>MDDANSSDSKVLNVWAMGDEAKSLKELAQKFTKDTGIEVKVQVIPWANAHDKLLTAVASKSGPDVVQMGTTWMPEFVEAGALLDITKDVEKSKNMNSDLFFPGSVKTTQFDGKTYGVPWYAETRVLFYRTDLLKKVGYNEAPKTWDELSDAALKLSKRGKDMYGFAIDPNEQTTGFIFGRQNGSPLFDKDGTPVFNKKPFVDTVTYLDSFIKNGSAPDTDLGLDASQSFGGDGIVPMFMSGPWMVNTLKDTAPDIDGKWATAVLPKKENNESSLGGANLSIFKYSNKKDDALKFMDYMSQPDVQL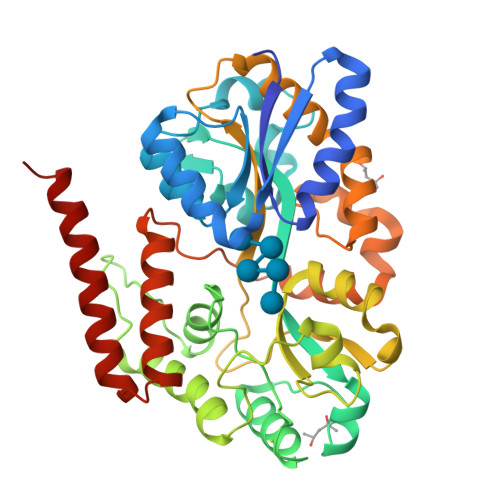SWLKDTNSMPARMDAWEDDMLKNDPYYKVFGEQMKTAEPMPLIPQFEEIAQLYGKSWEQIYRGGADVQTQMDTFNDQVEALLKKLEHHHHHH[2x]(2S)-2-{[1-(3-chloropyridin-2-yl)-1H-pyrazolo[3,4-d]pyrimidin-4-yl]oxy}-N-(5-methylpyridin-2-yl)-3-(propan-2-yloxy)propanamide 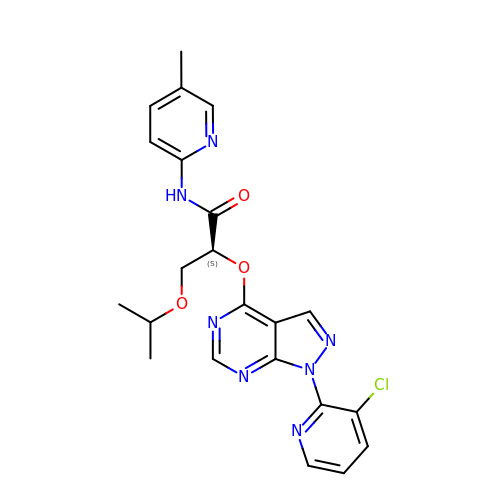| C22 H22 Cl N7 O3 | AAGISEXHOPCAHZ-KRWDZBQOSA-N>[4x]GPGSEFELRRQASNYQLTLTNTRATVNILMERLKKSDADVEQYRAELESVQLAKGALEQSYLVLQADAEQLRQQLTESQDALNALRSSSQTLQSE;>GPGSMKEQLLYLSKLLDFE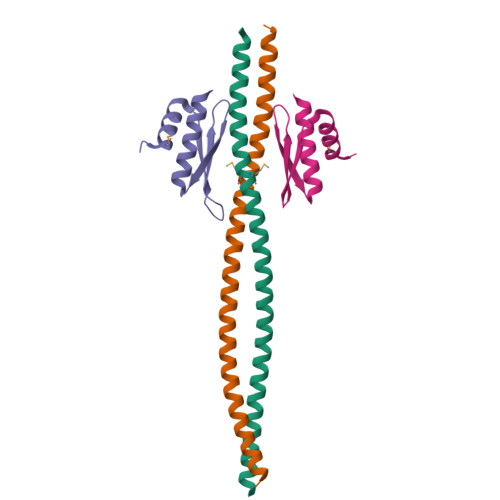VNFSDYPKGNHNEFLTIVTLSTHPPQICHGVGKSSEESQNDAASNALKILSKL[4x]> XSYLGKVYSLVKQENFDGFLKSAGLSDDKIQALVSDKPTQKMEANGDSYSNTSTGGGGAKTVSFKSGVEFDDVIGAGDSVKSMYTVD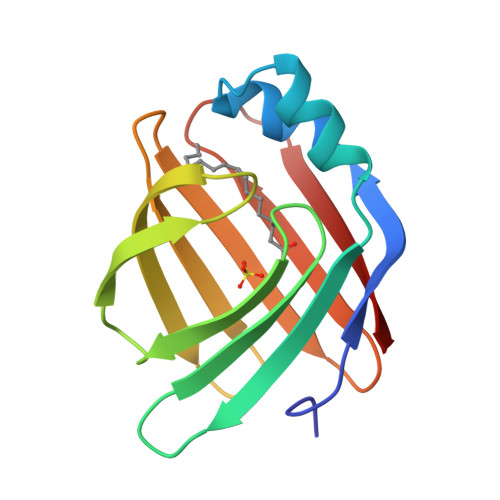GNVVTHVVKGDAGVATFKKEYNGDDLVVTITSSNWDGVARRYYKA> APKAPADGLKMDKTKQPVVFNHSTHKAVKCGDCHHPVNGKEDYQKCATAGCHDNMDKKDKSAKGAYHAMHD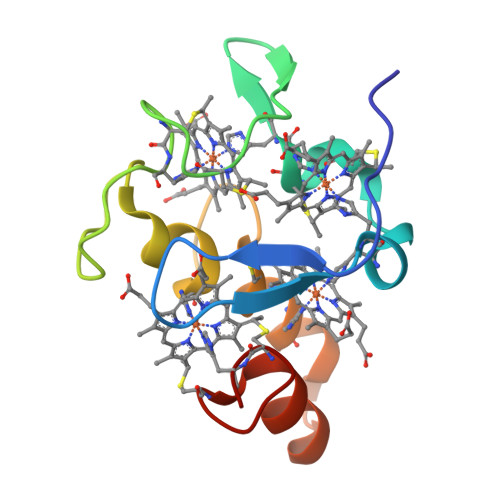KGTKFKSCVGCHLETAGADAAKKKELTGCKGSKCHS>[2x]SNANDLLPPEKAFVPELAVADDGVNVRFRIADGYYMYQAKIVGKTDPADLLGQPSFSKGEEKEDEFFGRQTVYHHEAQVAFPYAKAVGEPY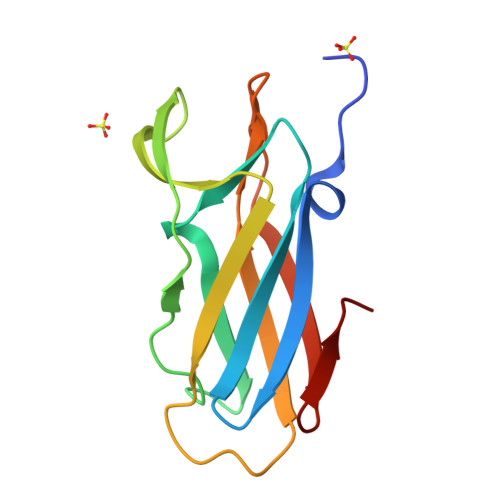KLVLTYQGCAEVGVCYPPVDTEFDISGNGTYHPQ SHIKIMATE-3-PHOSPHATE | C7 H11 O8 P | 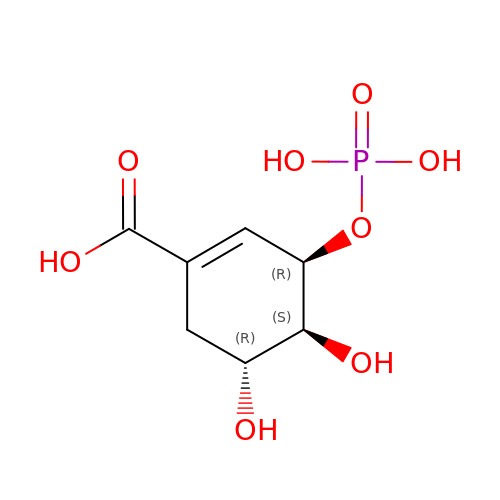QYOJSKGCWNAKGW-PBXRRBTRSA-N> MKHYALLISFLALSACSQGSEDLNEWMAQTRREAKAEIIPFQAPTLPVAPVYSPPQLTGPNAFDFRRMETDKKGENAPD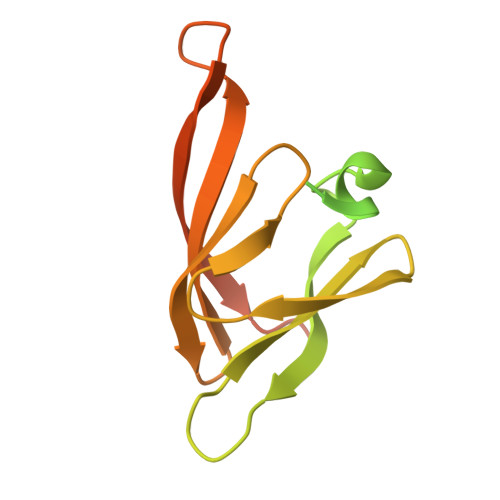TKRIKETLEKFSLENMRYVGILKSGQKVSGFIEAEGYVYTVGVGNYLGQNYGRIESITDDSIVLNELIEDSTGNWVSRKAELLLNSSDKNTEQAAAPAAEQN> GPGYLDSLGREAKCYSELNGCTKIYDPVCGTDGNTYPNECVLCFENR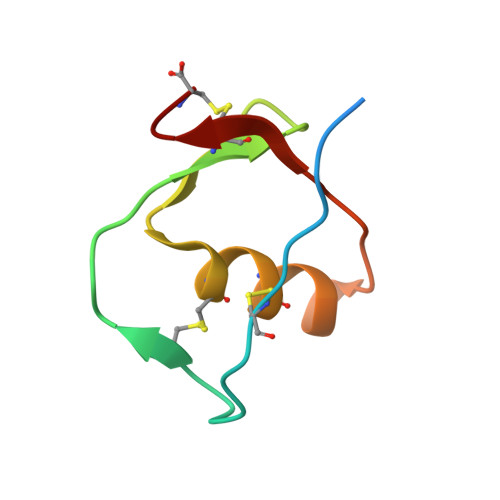KRQTSILIQKSGPC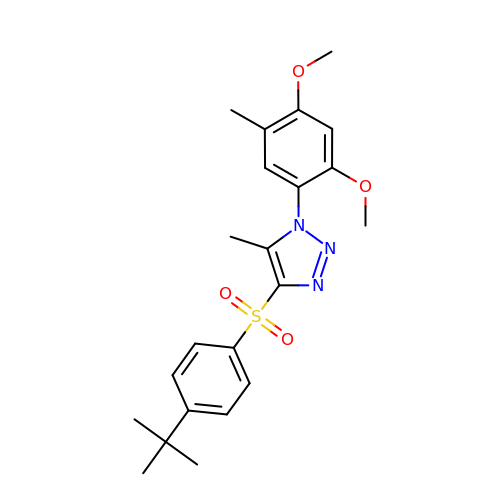4-[(4-tert-butylphenyl)sulfonyl]-1-(2,4-dimethoxy-5-methylphenyl)-5-methyl-1H-1,2,3-triazole | C22 H27 N3 O4 S | HXRSXIPYPZGCEK-UHFFFAOYSA-N> 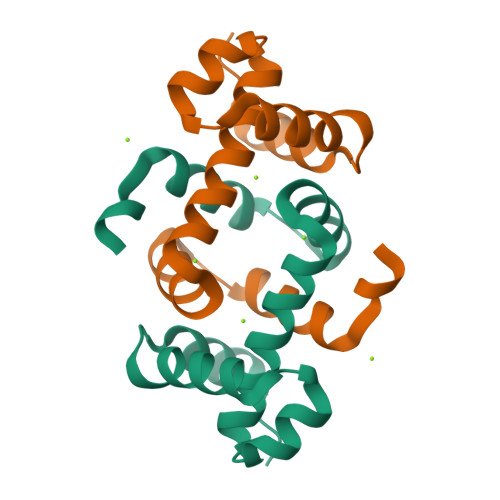MNNKLKTQAVEQLFQAILSLKDLDEAYDFFEDVCTINEILSLSQRFEVAKMLREHRTYLDIAEKTGASTATISRVNRSLNYGNDGYDRVFERLGMLEKESEDNK> GPLPKPTLWAEPGSVISWGNSVTIWCQGTLEAREYRLDKEESPAPWDRQNPLEPKNKARFSIPSMTEDYAGRYRCYYRSPVGWSQPSDPLELVMTGAYSKPTLSALPSPL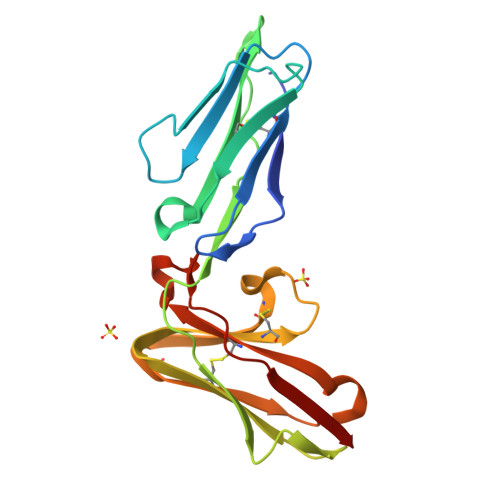VTSGKSVTLLCQSRSPMDTFLLCKERAAHPLLCLRSEHGAQQHQAEFPMSPVTSVHGGTYRCFSSHGFSHYLLSHPSDPLELIVSG>SQTVHFQGNPVTVANSIPQAGSKAQTFTLVAKDLSDVTLGQFAGKRKVLNIFPSIDTGVCAASVRKFNQLATEIDNTVVLCISADLPFAQSRFCGAEGLNNVITLSTFRNAEFLQAYGVAIADGPLKGLAARAVVVIDENDNVIFSQLVDEITTEPDYEAALAVLKA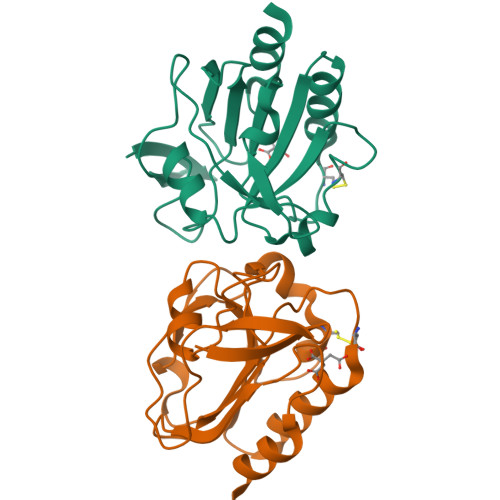[2x]> SDSLSKSPENWMSKLDDGKHLTEINIPGSHDSGSFTLKDPVKSVWAKTQDKDYLTQMKSGVRFFDIRGRASADNMISVHHGMVYLHHELGKFLDDAKYYLSAYPNETIVMSMKKDYDSDSKVTKTFEEIFREYYYNNPQYQNLFYTGSNANPTLKETKGKIVLFNRMGGTYIKSGYGADTSGIQWADNATFETKINNGSLN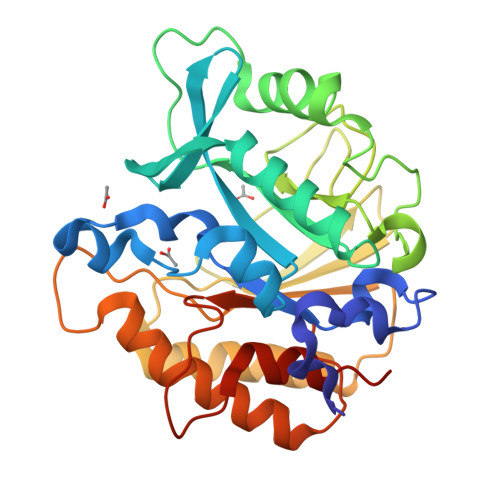LKVQDEYKDYYDKKVEAVKNLLAKAKTDSNKDNVYVNFLSVASGGSAFNSTSNYASHINPEIAKTIKANGKARTGWLIVDYAGYTWPGYDDIVSEIIDSNKLEHHHHHH>[6x]MARKTKVTPDDNSIIDLGPRVQSLMEQLATTKLEEGVKNLDMGSVYEITTVMVLGNSILGFHKGDLVKMVRPSVSARDLIGVGYATASAAVVRQRLIEHKIEAGAELIISGTAGGKTVLTNHYAAQMCAKGLKVAVVSMAEAERPLYGSVLHVFAALHLAAVSDVDVLYVDSLRSVYNELGGNLKKGGVSRQVDGMLTALDQYARAVNMRVVFTLNPSDDENVDAAVRSVFKTAS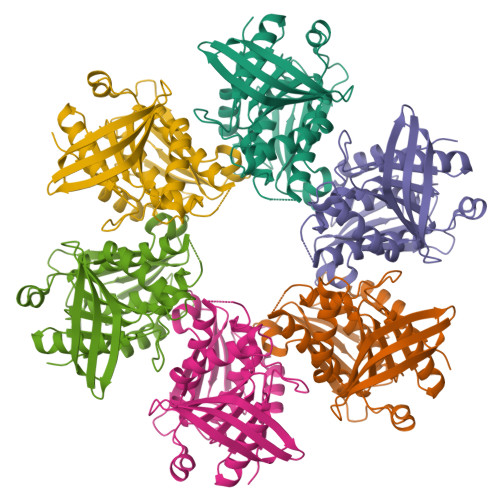ASMHTARRIKSFAVNGTAFTAETEIHLRADRSNSANRVSGDLVSR>[7x]MEQTQKLKLNLQHFASNNVKPQVFNPDNVMMHEKKDGTLMNEFTTPILQEVMENSKIMQLGKYEPMEGTEKKFTFWADKPGAYWVGEGQKIETSKATWVNATMRAFKLGVILPVTKEFLNYTYSQFFEEMKPMIAEAFYKKFDEA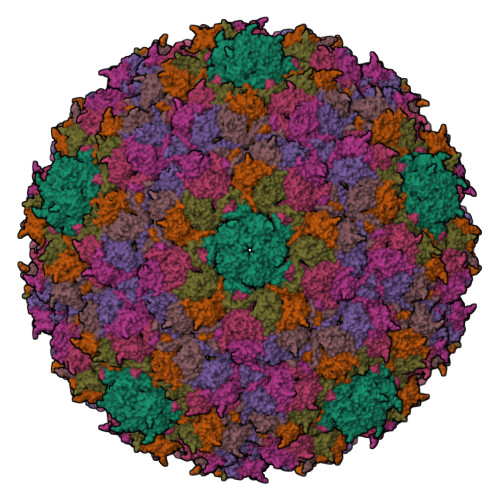GILNQGNNPFGKSIAQSIEKTNKVIKGDFTQDNIIDLEALLEDDELEANAFISKTQNRSLLRKIVDPETKERIYDRNSDSLDGLPVVNLKSSNLKRGELITGDFDKLIYGIPQLIEYKIDETAQLSTVKNEDGTPVNLFEQDMVALRATMHVALHIADDKAFAKLVPADKRTDSVPGEV;>MEENKLKFNLQFFADQSDDPDEPGGDGKKGNPDKKENDEGTEITFTPEQQKKVDEILERRVAHEKKKADEYAKEKAAEAAKEAAKLAKMNKDQKDEYEREQMEKELEQLRSEKQLNEMRSEARKMLSEAEVDSSDEVVNLVVTDTAEQTKSNVEAFSNAVKKAVNEAVKVNARQSPLTGGDSFNHSTKNKPQNLAEIARQKRIIKN[7x]> SDAMTTFLQRDEFAVTARVLGALFYYSPESHETAPLVQALLNDDWQAQWPLDAEALAPVAAMFKT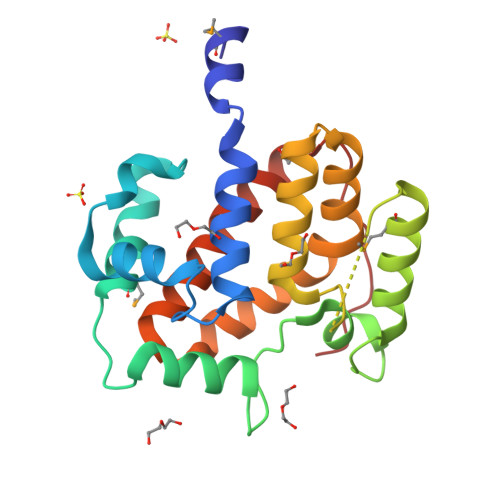HSEESLPQAWQRLFIGPYALPSPPWGSVWLDRESVLFGDSTLALRQWMRENGIQFEMQQNEPEDHFGSLLLLAAWLAENDRHHECEQLLAWHLFPWSSRFLDVFIDHAGHPFYQALGQLARLTLAQWQAQLIIPVAVKPLFR>[4x]MADEVILLDFWPSMFGMR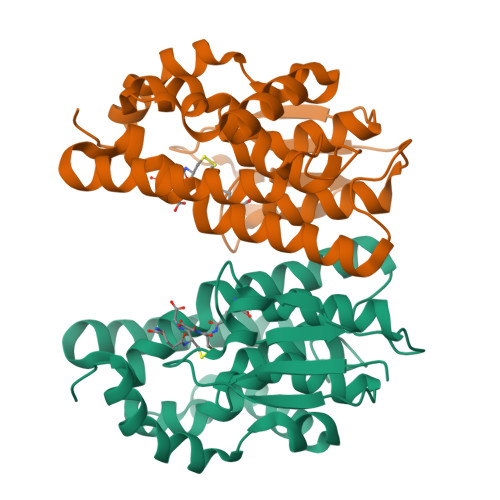TRIALEEKNVKFDYREQDLWNKSPILLEMNPVHKKIPVLIHNGNPVCESLIQIEYIDEVWPSKTPLLPSDPYQRAQAKFWGDFIDKKVYASARLIWGAKGEEHEAGKKEFIEILKTLESELGDKTYFGGETFGYVDIALIGFYSWFEAYEKFGSFSIEAECPKLIAWGKRCVERESVAKSLPDSEKIIKFVPELRKKLGIEIE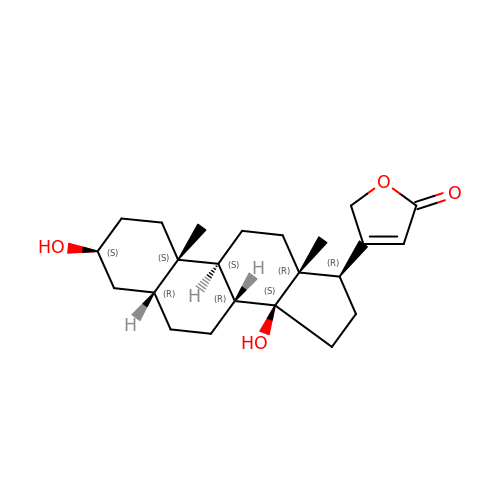DIGITOXIGENIN | C23 H34 O4 | XZTUSOXSLKTKJQ-CESUGQOBSA-N> MVKTFYITAAPVGAVPKFLDPLEPKFIPHALLELLPADRREATIKALEANGWEAVPAGGIVREYGYDAPIDLTDYDGAPASATVHDALRNNGWTPSGSVWHRTQTSPSLAQPPLITRNTLERLSSVDLVRQIVLQLTTFGWTATEDGSLTWAHDRIHTYLSPDFVERMRADNAAVLDSLFENGWRMCGAGHWQPGKARSPYLPITANGIVDASREALREGAAVVHLHTRATDDQATLAIPGLNTPIGIGSQRNHIVLDDYDRIMPTLLDLEPSAILNLSTSARGDRRASQSPLRRAHLKRYGHAQLAPDVASFSPGPVVFQAGGGYDNPNAFLADQLAHFAEVGVRPEIEVFNHTIVENSVTLYQSPLVKAGVPVLFMLVAAVDQYHRDPVSGDTSDDSLIDVPTRKAIAKLLQAGTDDAHEKAVELAATQLRPTVEKLRDNFPSCKISLLLPGPFQALLVDVAIALDLDGIRVGLEDALNVFDARVPGGVRKACGTGDQVRWLRRELERRGIGIVDAETLRDELGMSRPDVALFRQAEAALAHYPADERLVSADTILDALHPIVDTYRKIEDRLAAHLASAESLPADPAALAEHVLTAARSFGITIRSFVEELDRYEDHEYLVARYIQIPQALNFARELLVPRGYSIEAYDRALEDYARPGKTVTREHASYSVRVDQFKPLPLRCLEYLVGIPCRYNSDYSNVVNLGLRQSPRYSATMALLYHALRELTLELRDRSNASRKACGPLWTVLETPADASEPPVRRDVAPDEL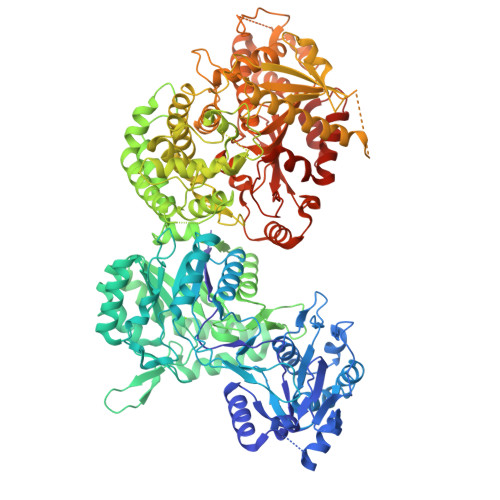AAAIASVDWVVLPSTPTTNYPLGIKLSNGMAQLFHGFVAQIAADPTLRPSRQTRRDTPLRLLAITHSGRRDDGETVIEASMLHNRFALNADPSGIYFSEESQLIYERLILPRLVDKPAKLAYTERQLVRRDAAGFPLYQDGARARRINAEQIERLPLLKCFAHSSGIATAQQLDVQACRDGERLGLTGDELRAFFDRALLVSFGSAADIHLDWLGTSVVDVTAFNDVRSLAGTTSRHYVIQPGEHADVLQHCLVHTQPADYRYDHATPVWQDGRQGKIVARLTGVFLLDDHARLDDGHSIRRYLAASPLWLRQWIARFHDAPADTGAHAILRELQSSMTDYRSSANQTTRRALA>AQVPASGKLLVDPRYSTNDQEESILQDIITRFPNVVLMKQTAQLRAMMTIIRDKETPKEEFVFYADRLIRLLIEEALNELPFQKKEVTTPLDVSYHGVSFYSKICGVSIVRAGESMESGLRAVCRGVRIGKILIQRDETTAEPKLIYEKLPADIRERWVMLLDPMCATAGSVC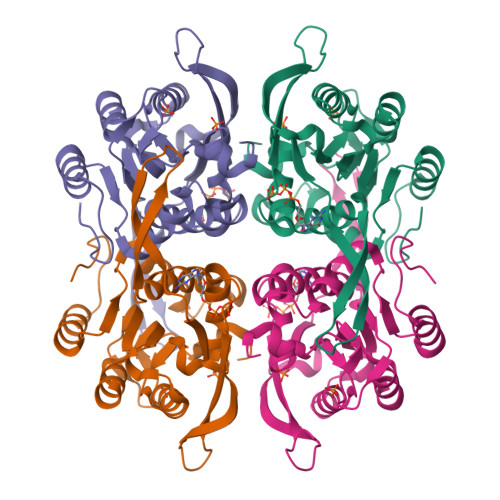KAIEVLLRLGVKEERIIFVNILAAPQGIERVFKEYPKVRMVTAAVDICLNSRYYIVPGIGDFGDRYFGTM[4x]>MKLKTTLFGNVYQFKDVKEVLAKANELRSGDVLAGVAAASSQERVAAKQVLSEMTVADIRNNPVIAYEDDCVTRLIQDDVNETAYNQIKNWSISELREYVLSDETSVDDIAFTRKGLTSEVVAAVAKICSNADLIYGAKKMPVIKKANTTIGIPGTFSARLQPNDTRDDVQSIAAQIYEGLSFGVGDAVIGVNPVTDDVENLSRVLDTIYGVIDKFNIPTQGCVLAHVTTQIEAIRRGAPGGLIFQSICGSEKGLKEFGVELAMLDEARAVGAEFNRIAGENCLYFETGQGSALSAGANFGADQVTMEARNYGLARHYDPFIVNTVVGFIGPEYLYNDRQIIRAGLEDHFMGKLSGISMGCDCCYTNHADADQNLNENLMILLATAGCNYIMGMPLGDDIMLNYQTTAFHDTATVRQLLNLRPSPEFERWLESMGIMANGRLTKRAGDPSLFF[2x];>MDQSSHHHHHHMDQKQIEEIVRSVMASMGQAAPAPSEAKCATTNCAAPVTSESCALDLGSAEAKAWIGVENPHRADVLTELRRSTVARVCTGRAGPRPRTQALLRFLADHSRSKDTVLKEVPEEWVKAQGLLEVRSEISDKNLYLTRPDMGRRLCAEAVEALKAQCVANPDVQVVISDGLSTDAITVNYEEILPPLMAGLKQAGLKVGTPFFVRYGRVKIEDQIGEILGAKVVILLVGER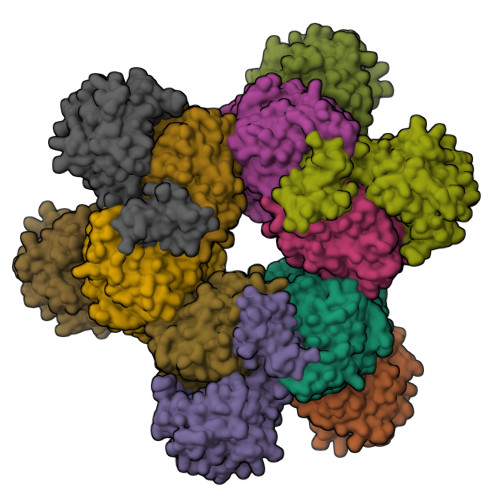PGLGQSESLSCYAVYSPRMATTVEADRTCISNIHQGGTPPVEAAAVIVDLAKRMLEQKASGINMTR[2x]>MSIHVNEANLTFHLQTDHTSYIFQIMKNGEAGQIYYGPRIHVQPTYQNLMSQEWRDATPSLNEENPNFQPATIKAEYASLGKGDFRQPAFQVTQANGSRITELTYDHYQLLTGKQRLANLPSTFDDTDDDAQTLVVSFNDRITGLALDLNYSIFPHQDVIVKSAKFTNPSSEKLVLNRALSSQLDLPDANYDLIQFSGTWARERHLYRHPLRPGMQSISSLRMASSHQQNPFMMLARPQTTDEQGAVFGFNLVYSGNFLDAIEVDQYSTSRILTGINPDEFGWNLAPQATFQTPEAILSYTSAGMNQLSQQMASFYQQHLVNPRFAHEERPVLINNWEATYFDFNEAKLMTIVNQAKRLGIEMFVLDDGWFGHRDDDTTSLGDWFVDQRKFPDGIEHFSQAVHQQGMKFGLWFEPEMVSVDSDLYQQHPDWLIHAPKSTPTPGRHQFVLDMARPEVVDYLFKLMSQMIESANLDYIKWDMNRYATEMFSSRLTSDQQLELPHRYILGVYQLYARLTQAYPNVLFESCASGGGRFDLGMMYYAPQAWTSDDTDAAERLLIQFGTSYGYPQAMMGAHVSAVPNDQMGRITSLKTRGAVAFFGDLGYELDITKMAPTELDQVKKQVAFYKCYRQLFQFGKFYRIDSPFVEDGNVTSWQVVSDDQKQAIAARYQLLNHPNAPYTRFYFKGLRPNQRYQINDDP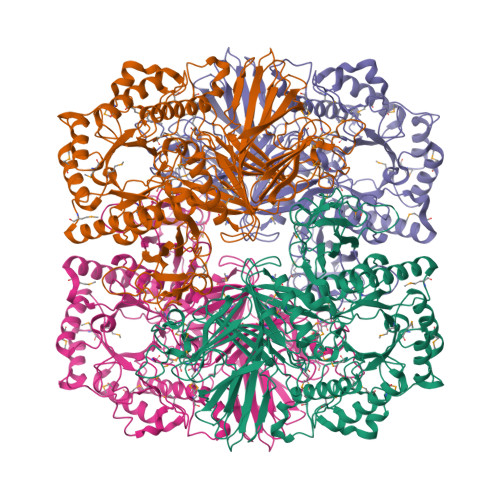STYYGDELMNAGYFVPTILADGQESKDFYTQLFVVTAILEHHHHHH[4x]[({5-[4-(propan-2-yloxy)phenyl]pyridin-3-yl}amino)methanediyl]bis(phosphonic 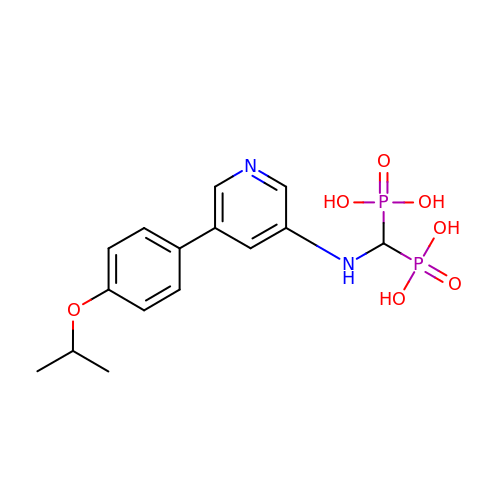acid) | C15 H20 N2 O7 P2 | AEYMCQCOKHXTEC-UHFFFAOYSA-N> MRSYLILRLAGPMQAWGQPTFEGTRPTGRFPTRSGLLGLLGACLGIQRDDTSSLQALSESVQFAVRCDELILDDRRVSVTGLRDYHTVLG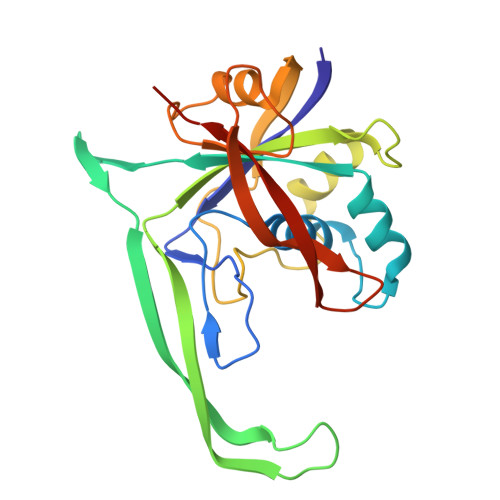AREDYRGLKSHETIQTWREYLCDASFTVALWLTPHATMVISELEKAVLKPRYTPYLGRRSCPLTHPLFLGTCQASDPQKALLNYEPVGGDIYSEESVTGHHLKFTARDEPMITLPRQFASREWYVIKGGMDVSQ>CATGTRQSPINIQWKDSVYDPQLAPLRVSYDAASCRYLWNTGYAFQVEFDDSCEDSGISGGPLGNHYRLKQFHFHWGATDEWGSEHAVDGHTYPAELHLVHWNSTKYENCKKASVGENGLAVIGVFLKLGAHHQALQKLVDVLPEVRHKDTQVAMGPFDPSCLMPACRDYWTYPGSLTTPPLAESVTWIVQKTPVEVSPSQLSMFRTLLFSGRGEEEDVMV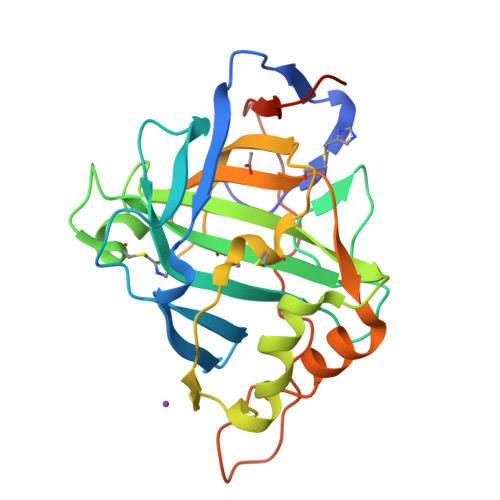NNYRPLQPLRDRKLRSSFRLDRTKMRS[2x]> MTMMDMNFKYCHKIMKKHSKSFSYAFDLLPEDQRKAVWAIYAVCRKIDDSIDVYGDIQFLNQIKEDIQSIEKYPYEYHHFQSDRRIMMALQHVAQHKNIAFQSFYNLIDTVYKDQHFTMFETDAELFGYCYGVAGTVGEVLTPILSDHETHQTYDVARRLGESLQLINILRDVGEDFENERI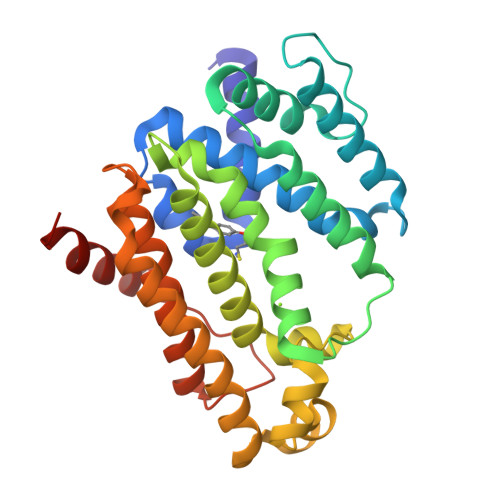YFSKQRLKQYEVDIAEVYQNGVNNHYIDLWEYYAAIAEKDFRDVMDQIKVFSIEAQPIIELAARIYIEILDEVRQANYTLHERVFVEKRKKAKLFHEINSKYHRI> KGSVVIVGRIILS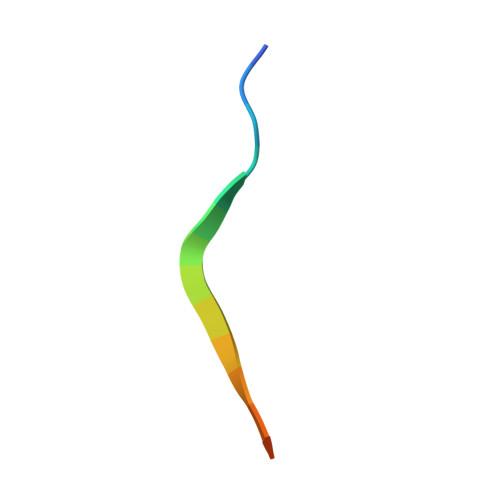GRK> MSNLSGTDKSVILLMTIGEDRAAEVFKHLSTREVQALSTAMANVRQISNKQLTDVLSEFEQEAEQFAALNINANEYLRSVLVKALGEERASSLLEDILETRDTTSGIETLNFMEPQSAADLIRDEHPQIIATILVHLKRSQAADILALFDERLRHDVMLRIATFGGVQPAALAELTEVLNGLLDGQNLKRSKMGGVRTAAEIINLMKTQQEEAVITAVREFDGELAQKIIDEMFLFENLVDVDDRSIQRLLQEVDSESLLIALKGAEPPLREKFLRNMSQRAADILRDDLANRGPVRLSQVENEQKAILLIVRRLAETGEMV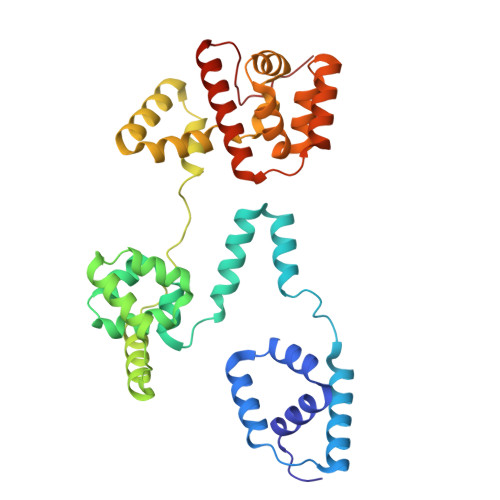IGSGEDTYV> TKWDLPTAYPASNLHVENLTQFVKDVDSLSGGKLKITLHNNASLYKAPEIKRAVQGNQAQIGEILLTNFANEDPVYELDGLPFLATGYDASFKLYQAQKPFLEKKLASQGMMLLYSVAWPPQGIFANRDIKQVSDMKGLKWRAYSPVTAKIAELVGAQPVTVQQAELAQAMATGVIDSYMSSGSTGFDTKTYEYIKKFYDTEAWLPKNAVLVNKKAFDALDPAT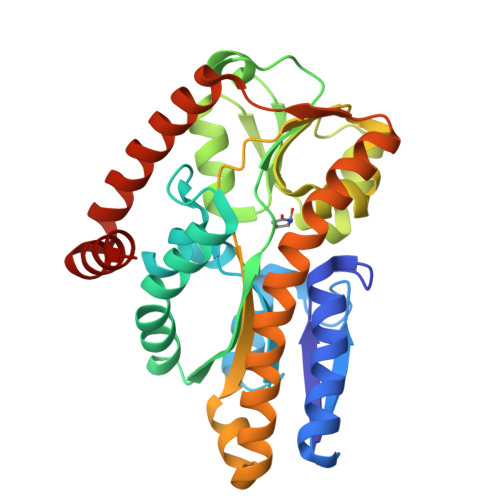QQALKKAGAQAEERGWKLSQEKNSWYKEQLAKNGMAIIAPTAELKSGLTEVGKRMLDDWLKKAGADGQAMIDAYRKQ> MRFGFLLNEVLTGFRRNVTMTIAMIL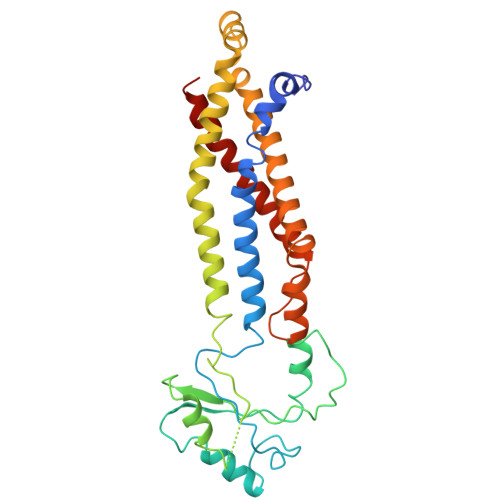TTAISVGLFGGGMLVVRLADSSRAIYLDRVESQVFLTEDVSANDSSCDTTACKALREKIETRSDVKAVRFLNRQQAYDDAIRKFPQFKDVAGKDSFPASFIVKLENPEQHKDFDTAMKGQPGVLDVLNQKELIDRLFAVLDGLSNAAFAVALVQAIGAILLIANMVQVAAYTRRTEIGIMRLVGASRWYTQLPFLVEAMLAATMGVGIAVAGLMVVRALFLENALNQFYQANLIAKVDYADILFITPWLLLLGVAMSGLTAYLTLRLYVRR> GPHMKSTFKSEYPFEKRKAESERIADRFPNRIPVICEKAEKSDIPEIDKRKY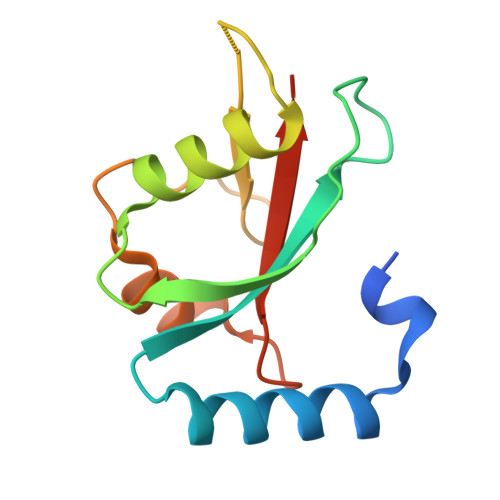LVPADLTVGQFVYVIRKRIMLPPEKAIFIFVNDTLPPTAALMSAIYQEHKDKDGFLYVTYSGENTFG> HKCDITLQEIIKDLNSLTEQKTLCTELTVTDIFAASKNTTEKETFCRAATVLRQFYSHHEKDTRCLGATAQQFHRHKQLIRDLKRLDRNLWGLAGLNSCPVKEANQSTLENFLERLKTIMREKYSKCSS

Interleukin 4 (IL-4) is a pleiotropic cytokine that plays a major regulatory role in the immune system. Signal transduction of IL-4 is mediated by a sequential binding process, initiated first by binding of IL-4 to its high-affinity single membrane spanning receptor chain IL-4Rα. This intermediate ligand receptor complex then recruits one of two possible low-affinity receptor subunits, the common gamma chain (γc) or the IL-13Rα1 chain, into the functional hetero-trimeric complex to initiate signalling. The overall structure of IL-4 comprises the known four-helical bundle in up-up-down-down topology, which like the crystal packing is unaffected by these mutations.

To determine whether the stabilizing effects of the two single mutations T13D and F82D might act in a cooperative manner, we generated the IL-4 double variant T13D-F82D, which we expected to bind IL-4Rα with a KD in the sub-picomolar range. However, interaction analysis revealed that the apparent KD of the complex between IL-4Rα and this IL-4 variant is higher than that observed for the individual single mutation variants T13D and F82D and is similar to that for wild-type IL-4. In addition, the kinetic rate constants, especially the dissociation rate, clearly reflect the binding characteristics of wild-type IL-4. The structures of the IL-4 variants T13D (max. resolution 1.65 Å), F82D (max. resolution 1.7Å) and T13D-F82D (max. resolution 1.8Å) were refined on the basis of the structure of wild-type IL-4 (max. resolution 1.8Å); all crystals were obtained under identical conditions, allowing detailed comparison. In the case of the double variant, T13D-F82D, the side chain of Arg85 also occupies a different side chain conformation from that in wild-type IL-4. Although two "acceptor" carboxylate groups are present, Asp13 and Asp82, the side chain of Arg85 exhibits only one defined side chain conformation in which the guanidinium group is hydrogen bonded to the carboxylate group of Asp82. As in variant F82D, the temperature factors of the side chain atoms of Arg85 are elevated compared to main chain atoms. The fixation of the side chain of Arg85 to the core structure of IL-4 might therefore be not as strong as observed for T13D. Although only a single defined side chain conformation for Arg85 is observed in T13D-F82D, the loss in affinity of the double variant compared to both super-agonists might result from a competition between two possible side chain conformations of Arg85. Since the additional interaction is mediated in both super-agonists by the same indirect mechanism via Arg85, this also explains why combination of two super-agonistic mutations did not lead to a further increase in binding affinity.At the cell division site, FtsZ protofilaments form a highly dynamic, membrane-bound structure, the Z-ring, which serves as a scaffold for the recruitment of the extra-cytoplasmic cell wall biosynthetic machinery. Here we investigate the physiological function of Corynebacterium glutamicum SepF, the only cell division-associated protein from Actinobacteria known to interact with the conserved C-terminal tail of FtsZ. Our structural data revealed the FtsZ-binding pocket, defining the SepF homodimer as the functional unit, and suggesting a reversible β-sheet-mediated oligomerization interface possibly regulated via an alpha helical switch. We found that FtsZ filaments and lipid membranes have opposing effects on SepF polymerization, pointing to a complex dynamic role of the protein at the division site, involving FtsZ bundling, Z-ring tethering and membrane reshaping activities that are needed for proper Z-ring assembly and function.

To further investigate this hypothesis, we removed the helix and crystallized the resulting SepFΔML,Δα3 construct alone and in complex with FtsZCTD. Despite a different crystal packing, the two structures did show a dimer-dimer association mediated by the opposing β-sheets in the crystal, generating linear SepF polymers similar to those observed for the B. subtilis homolog. These observations demonstrate that the β-sheet is indeed prone to self-interaction in solution and suggest that the amphipathic helix α3 might regulate SepF polymerization. In our hands, C. glutamicum SepF devoid of helix α3 (i.e., with the β-sheet accessible for protein–protein interactions) remained dimeric in solution and we were unable to detect higher order assemblies by size exclusion chromatography or analytical ultracentrifugation.

>[2x]MSYQSTIVPVELHSFEDAQVIGGAFRDGDAVVFDMSLLSREEARRIVDFAAGLCFALRGKMQKIDSVTFAVVPE> GSMVEATAQETDRPRFSFSIAAREGKARTGTIEMKRGVIRTPAFMPVGTAATVKALKPETVRATGADIILGNTYHLMLRPGAERIAKLGGLHSFMGWDRPILTDSGGYQVMSLSSLTKQSEEGVTFKSHLDGSRHMLSPERSIEIQHLLGSDIVMAFDESTPYPATPSRAASSMERSMRWAKRSRDAFDSRKEQAENAALFGIQQGSVFENLRQQSADALAEIGFDGYAVGGLAVGEGQDEMFRVLDFSVPMLPDDKPHYLMGVGKPDDIVGAVERGIDMFDSVLPTRSGRNGQAFTWDGPINIRNARFSEDLKPLDSECCCAVCQKWSRAYIHHLIRAGEILGAMLMTEHNIAFYQQLMQKIRDS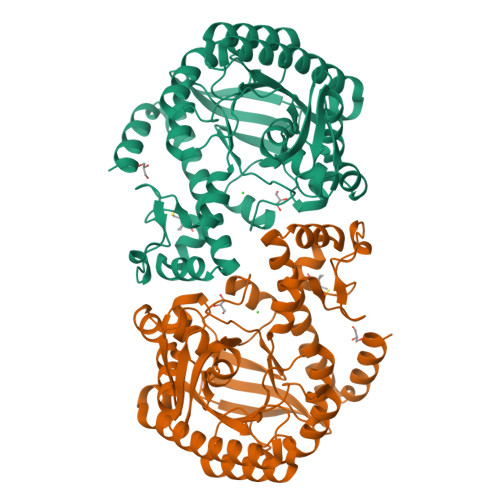ISEGRFSQFAQDFRARYFARNS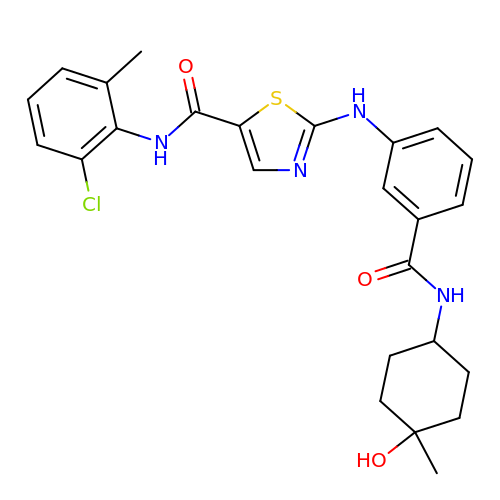(2~{Z})-~{N}-(2-chloranyl-6-methyl-phenyl)-2-[3-[(4-methyl-4-oxidanyl-cyclohexyl)carbamoyl]phenyl]imino-1,3-thiazolidine-5-carboxamide | C25 H27 Cl N4 O3 S | FJOOAAAPKODUJU-QFMRLBMFSA-N> ADQPSPTWGIDRIDQRNLPLDNNYHTDYDGSGVTAFVIDTGVLNTHNEFGGRASSGYDFIDNDYDATDCNGHGTHVAGTIGGSTYGVAKNVNVVGVRVLNCSGSGSNSG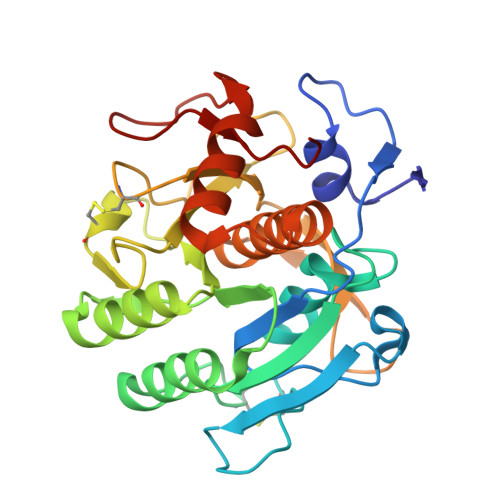VIAGINWVKNNASGPAVANMSLGGGASQATDDAVNAAVAAGITFVVAAGNDNSNACNYSPARAADAITVGSTTSNDSRSSFSNYGTCLDIYAPGSSITSSWYTSNSATNTISGTSMASPHVAGVAALYLDENPNLSPAQVTNLLKTRATADKVTDAKTGSPNKLLFSLA NAMPT functions as a homo-dimeric enzyme that catalyzes the rate limiting step in the primary salvage pathway for NAD synthesis, the transfer of a phosphoribosyl residue from 5-phosphoribosyl-1-pyrophosphate (PRPP) to nicotinamide (NAM) to produce nicotinamide mononucleotide (NMN). Crystal structures of NAMPT in numerous ligand-bound forms have been reported. These structures consistently display a NAMPT homo-dimer with two essentially identical active sites at the dimer interface. Typical NAMPT inhibitors were found to occupy the portion of active site responsible for NAM binding and a tunnel-shaped cavity extending from the NAM binding site. Furthermore, we determine the crystal structures of six NAMPT mutants in the apo form and in complex with various inhibitors and present a definitive model to explain the differential effects of the mutations on various structural classes of NAMPT inhibitors.

The crystal structure of G217R in complex with APO866 revealed that the more flexible and narrower linker of APO866 adopted an alternative conformation but nonetheless could fit through the altered tunnel. G217R causes His191 side chain to rotate to the same extent as G217V, while introducing additional changes to the structure of the NAMPT inhibitor-binding site. The R217 side chain competes for space with the bound inhibitor (e.g., with the terminal phenyl-trifluoromethyl group of GNE-618) in a similar fashion as H191R. Besides introducing steric clashes, the R217 guanidinium group also creates a basic patch at the surrounding protein surface that favors polar groups over hydrophobic groups. We conclude that these additional structural changes render the G217R mutation more deleterious for NAMPT inhibitor binding across structural classes.

>[2x]MNPAAEAEFNILLATDSYKVTHYKQYPPNTSKVYSYFECREKKTENSKLRKVKYEETVFYGLQYILNKYLKGKVVTKEKIQEAKDVYKEHFQDDVFNEKGWNYILEKYDGHLPIEIKAVPEGFVIPRGNVLFTVENTDPECYWLTNWIETILVQSWYPITVATNSREQKKILAKYLLETSGNLDGLEYKLHDFGYRGVSSQETAGIGASAHLVNFKRTDTVAGLALIKKYYGTKDPVPGYSVPAAEHSTITAWGKDHEKDAFEHIVTQFSSVPVSVVSDSYDIYNACEKIWGEDLRHLIVSRSTQAPLIIRPDSGNPLDTVLKVLEILGKKFPVTENSKGYKLLPPYLRVIQGDGVDINTLQEIVEGMKQKMWSIENIAFGSGGGLLQKLTRDLLNCSFKCSYVVTNGLGINVFKDPVADPNKRSKKGRLSLHRTPAGNFVTLEEGKGDLEEYGQDLLHTVFKNGKVTKSYSFDEIRKNAQLNIELEAAHHLEHHHHHHHH> GSDNAEKGKVSNDDASVDFVAEPVK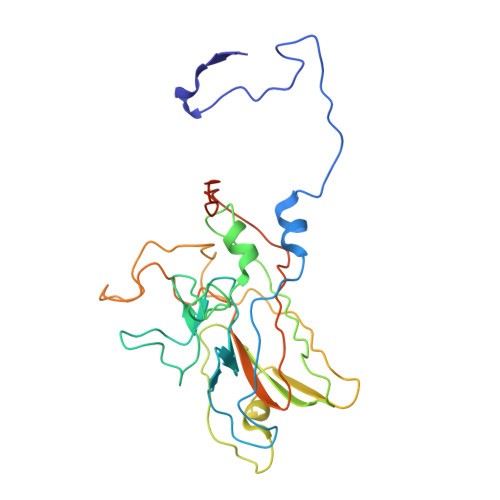LPENQTRVAFFYDRAVPIGMLRPGQNIESTFVYQENDLRLNCLLLTPLPSFCPDSTSGPVKTKAPVQWRWVRSGGTTNFPLMTKQDYAFLCFSPFTYYKCDLEVTVSALGTDTVASVLRWAPTGAPADVTDQLIGYTPSLGETRNPHMWLVGAGNTQISFVVPYNSPLSVLPAAWFNGWSDFGNTKDFGVAPNADFGRLWIQGNTSASVRIRYKKMKVFCPRPTLFFPWPVSTRSKINADNPVPILELE>[4x]MGSSFVYLPR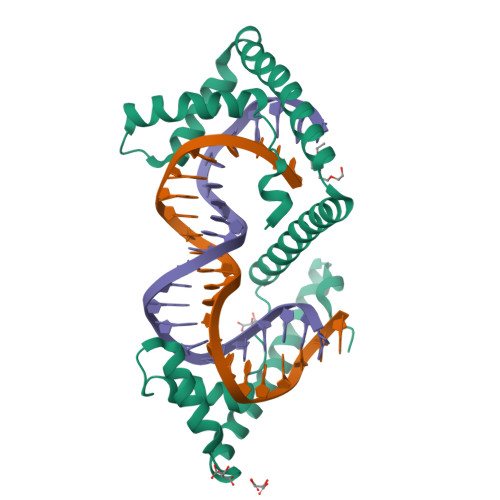WFSSVLASCPKKPVSSYLRFSKEQLPIFKAQNPDAKTTELIRRIAQRWRELPDSKKKIYQDAYRAEWQVYKEEISRFKEQLTPSQIMSLEKEIMDKHLKRKAMTKKKELTLLGKPKRPRSAYNVYVAERFQEAKGDSPQEKLKTVKENWKNLSDSEKELYIQHAKEDETRYHNEMKSWEEQMIEVGRKDLLRRTIKKQRKYGAEECLQHHHHHH>[2x]MPNIKIFSGSSHQDLSQKIADRLGLELGKVVTKKFSNQETCVEIGESVRGEDVYIVQSGCGEINDNLMELLIMINACKIASASRVTAVIPCFPYARQDKKDKSRAPISAKLVANMLSVAGADHIITMDLHASPIQGFFDIPVDNLYAEPAVLKWIREN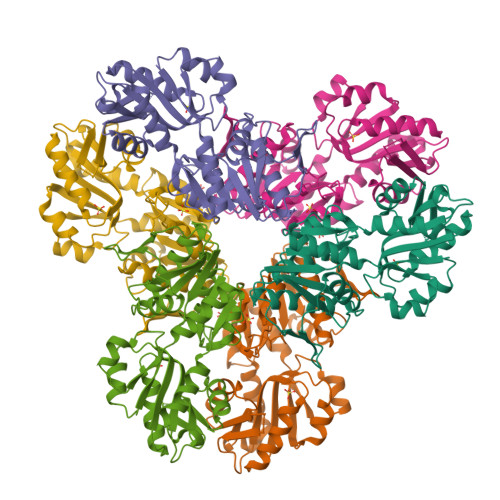ISEWRNCTIVSPDAGGAKRVTSIADRLNVDFALIHKERKKANEVDRMVLVGDVKDRVAILVDDMADTCGTICHAADKLLSAGATRVYAILTHGIFSGPAISRINNACFEAVVVTNTIPQEDKMKHCSKIQVIDISMILAEAIRRTHNGESVSYLFSHVPLLEHHHHHH>[6x]MGGSHHHHHHGDDDDKMVEFPEGFVWGAATSGPQTEGNFHKQHQNVFDYWFATEPEQFDAGVGPDTASNFYNDYDHDLALMAQAGVQGLRTSIQWTRLIDDFETASLNADGVAFYNHVIDS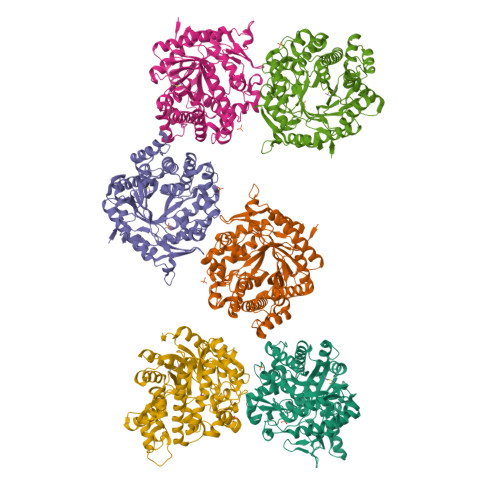MLAHHITPYINLHHFDLPVALYDKYHGWESKHVVELFVKFAEQCFKLFGDRVDHWYTFNEPKVVVDGQYLYGWHYPQVINGPKAVQVAYNMNLASAKTVARFHELCVRPEQQIGIILNLTPAYAASDDPADLAAAEFAELWSNNLFLDPAVLGHFPEKLVERLTMDGVLWDATPTELAIIAANPVDCLGVNYYHPFRVQRPDISPKSLQPWMPDIYFKEYDMPGRMMNVDRGWEIYPQAMTDIARNIQKNYGNIPWMISENGMGVAGEERFLDKQGVVQDDYRIDFMKEHLTALAKGIAAGSNCQGYFVWSGIDCWSWNHAYHNRYGLIRNDIHTQTKTLKKSAKWFAELGERNGF>[2x]SMKEFRPGDKVVLPPYGVGVVAGIAQRSVSGVSRAYYQVDFPGSRSKAYVPVEAPHSVGLRKALAPEEVPVILDLLKNGR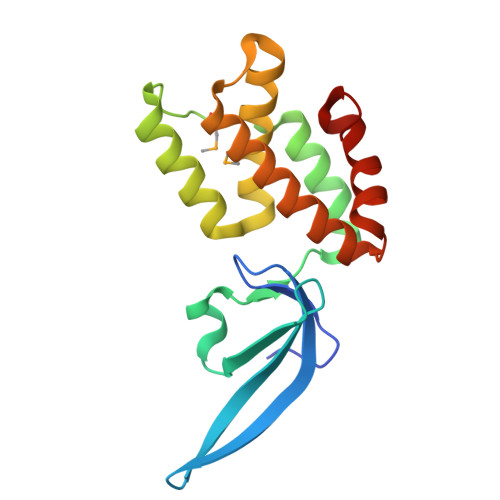MPLPKQWAARHRKTSEILADGNPYRIAQMAGQLRAWEVERGLPDLDRQALRRAIHLLAEEVAQSLEITVQEAKRLFEEAWGEELN> GGG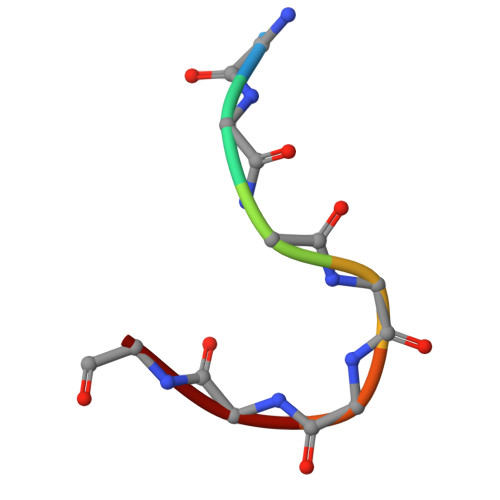GGGG In 2011, desmoglein-2 (DSG2), a component of desmosomes carrying four extracellular domains (EC1 to EC4) has been reported to be the main receptor of HAdV of serotype 3, 7, 11, and 14. The critical entry step in the viral cycle is mediated by the adenovirus trimeric fiber and more especially by its distal globular domain called the ‘knob’. In the present study, we investigate the binding mechanism of the ARD causing agent HAdV7 to the EC23 module of DSG2 using biochemical and biophysical methods. We report the atomic structure of the complex solved by cryo-EM using phase-plate providing improved high-contrast images.

HAd7K in complex with EC23 resulted in two coefficients at 6.9S and 9.7S, suggesting different stoichiometries. This hypothesis was confirmed by the cryo-EM analysis in which two populations corresponding to HAd7K with two or three modules were found. Extensive 3D classifications and refinements indeed show that the complex mainly exists in two forms, i.e., a HAd7K trimer can interact with two or three EC23 modules hereafter named HAd7K-(EC23)2 and HAd7K-(EC23)3, respectively. HAd7K-(EC23)2 and HAd7K-(EC23)3 were solved to 3.5 and 3.1 Å resolution, respectively, which allowed the fitting and refinement of two atomic models using the existing X-ray structures of HAd7K and EC23. The two models are very similar with the exception of the extra EC23 module in the HAd7K-(EC23)3 complex. The overall root mean square deviation (RMSD) between HAd7K-(EC23)2 and HAd7K-(EC23)3 (without the third EC23 module) is 0.5 Å. Each EC23 module interacts with two different monomers of the HAd7K. Furthermore, each EC domain (i.e., EC2 or EC3) interacts with one HAd7K monomer. For the EC3 domain, the main interacting residue is R316 which fits into a pocket formed by two loops at the surface of one HAd7K monomer. R316 forms putative hydrogen bonds and a salt bridge with D265 while the other HAd7K residues defining the pocket are F269 and V300.

>[3x]GSHMGLTFNSNNICIDDNINTLWTGVNPTTANCQIMASSESNDCKLILTLVKTGALVTAFVYVIGVSNDFNMLTTHKNINFTAELFFDSTGNLLTSLSSLKTPLNHKSGQNMATGALTNAKGFMPSTTAYPFNVNSREKENYIYGTCYYTASDHTAFPIDISVMLNQRALNNETSYCIRVTWSWNTGVAPEVQTSATTLVTSPFTFYYIREDD;>QGAMEVLDINDNEPVFTQDVFVGSVEELSAAHTLVMKINATDADEPNTLNSKISYRIVSLEPAYPPVFYLNKDTGEIYTTSVTLDREEHSSYTLTVEARDGNGEVTDKPVKQAQVQIRILDVNDNIPVVENKVLEGMVEENQVNVEVTRIKVFDADEIGSDNWLANFTFASGNEGGYFHIETDAQTNEGIVTLIKEVDYEEMKNLDFSVIVANKAAFHKSIRSKYKPTPIPIKVKVKNVKEGI[3x]>[4x]AAQSVDIHKDQIIFSEGDAGDCAYIIEKGRVLIYLTKDKEEIPLTILGEGEIFGEMALIDNQNRSASVRALEDVRLAIVTKQQVLERVSTADKVVQLLMRVLLKRLRRKNI

Herein, we provide high‐resolution structures for an EAL enzyme Bd1971, from the predatory bacterium Bdellovibrio bacteriovorus, which is controlled by a second signaling nucleotide, cAMP. The Bd1971 domain architecture is predicted to consist of an N‐terminal cNMP sensory domain (cyclic nucleotide monophosphate, postulated to bind cAMP or cGMP), a middle linker region, and C‐terminal catalytic EAL barrel. We reveal that regulation of c‐di‐GMP hydrolysis arises from a domain‐swapping of the “regular” cNMP fold, which undergoes significant rearrangements upon binding of stimulus, communicating a series of conformational changes over 40 Å to license a productive state at the EAL dimer interface. C‐di‐GMP turnover was increased ~8‐fold in the presence of cAMP or cGMP, further supporting the proposal that cNMPs are activators of Bd1971.

The negative co‐operativity of the Bd1971ΔEAL cNMP sensor dimer raised the prospect of a potentially stable (intermediary) state in which the protein could be half‐occupied by a single cAMP—this is important given that there is little to no structural information on any intermediary state for other cNMP sensors. In screening for cNMP‐bound Bd1971ΔEAL, lower concentrations of cAMP did indeed result in different crystal forms, and we were able to solve the structure of a half‐occupied dimer (hereafter referred to as Bd1971ΔEAL‐mid) to 2.79 Å resolution. This form has two dimers in the asymmetric unit, each binding a singular cAMP molecule, the fold traceable until the end of the C‐helix (residue 114). Strikingly, the conformational cNMP swing‐out between the apo and bound forms is replicated to an intermediary degree in the cAMP‐occupied chain of Bd1971ΔEAL‐mid, with a rotation of ~30° and translation (at β‐hairpin) of 10 Å (aligned via C‐helices which again do not shift relative to one another). Significantly, the empty sensor chain of Bd1971ΔEAL‐mid adopts the “fully outward” domain juxtaposition observed in both chains of the apo‐form. Using the distance between the Cα atoms of hinge residue Asp95 and small helix Ile62 as a measure of P‐loop migration, the Bd1971ΔEAL‐mid structure (16.7 Å) sits between that of the apo‐form (20.1 Å, swung out) and two‐site bound state (14.6 Å, swung in). The nucleotide‐bound pocket of Bd1971ΔEAL‐mid reveals cAMP to be bound in the syn conformation; of the two full‐length, bound‐state structures of Bd1971, this pose resembles the cGMP complex (syn) more closely than the cAMP complex (anti). The result of this difference between the different forms is that the full‐length complexes position the neighboring Arg108 residue (corresponding to the conserved hydrophobic cap in other cNMP sensors; Kornev et al, 2008) in an orientation that promotes full cNMP body:C‐helix closure (2.6–2.9 Å from the carbonyl of Ile55), whereas the Bd1971ΔEAL‐mid syn cAMP complex results in a kinked conformation of the Arg108 cap (5.15 Å away from Ile55), resulting in the partial domain closure observed.>[2x]MTAVRSESAELSQSPASYRFPPGFVWGAATAAYQIEGAAAEDGRTPSIWDTFSHTPGRVLNGDTGDIAADHYHRFRDDVALMSDLNLGAYRFSVSWSRVQPTGRGPAVQRGLDFYRQLVDELLEKGITPVATLYHWDLPQDLEDVGGWTVRDTPERFAEYTEIVAAALGDRVPYWTTLNEP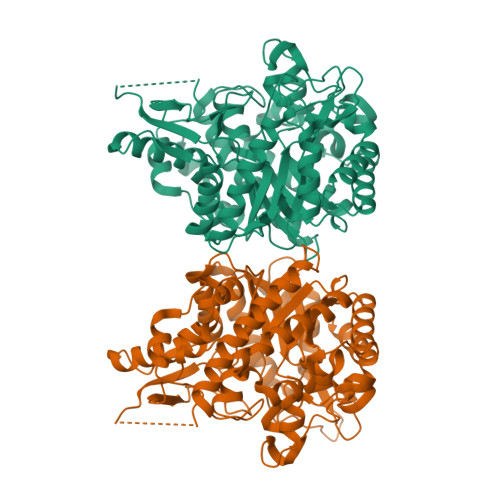WCSAYLGYGSGVHAPGRTDPEAALKAVHHLNLAHGRGIGVLRSLLPSTARTSITLNLHQIRPLSTSPADLDAARRIDAVGNRVWLGPILDGAYPQDVLADTGHLVDWDRLVRDGDLEEISRPIDLLGINYYTPTLVSDGRAHADGPAMPRNDGHGASAHSPWPGSEHVAFHLAPGETTAMRWAVDASGLYDLLMRIHREHPGLPMMVTENGAAYDDYISPEGAINDPDRIAYLRGHLSAVHRALADGADVRGYFLWSLLDNFEWAYGYSKRFGAVYVDFGTQRRIPKQSAHWYAAVARDNVLPDGPEEDGTS> PPGTVDKKMVEKCWKLMDKVVRLCQNPKLALKNSPPYILDLLPDTYQHLRTILSRYEGKMETLGENEYFRVFMENLMKKTKQTISLFKEGKERMYEENSQPRRNLTKLSLIFSHMLAELKGIFPSGLFQGDTFRITKADAAEFWRKAFGEKTIVPWKS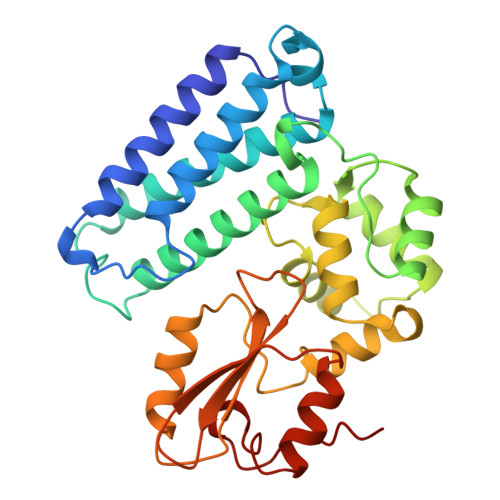FRQALHEVHPISSGLEAMALKSTIDLTCNDYISVFEFDIFTRLFQPWSSLLRNWNSLAVTHPGYMAFLTYDEVKARLQKFIHKPGSYIFRLSCTRLGQWAIGYVTADGNILQTIPHNKPLFQALIDGFREGFYLFPDGRNQNPDLTG> MRGSHHHHHHGRSGDDDDKMKVLNDLLGYKNRKLYQDNKMFNFTLDSVLVARFCNLNS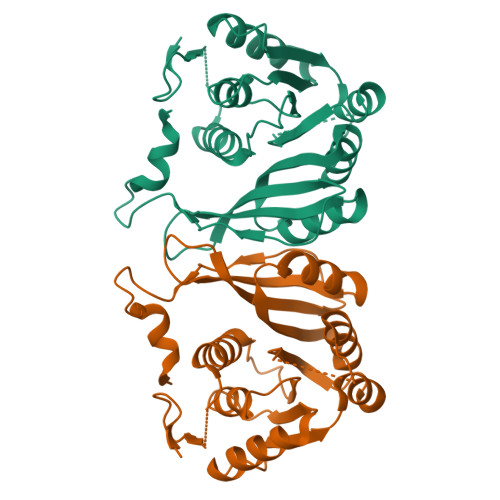KKKKICDFGTNNAVIPLILSKYTKAKIIGVEIQNKAVEIANENIKLNGLEDQIEIVHADIKEFSKLHNQEFDLVVCNPPFFKMDGNPKLKEISLEVANARHEILITLEDIIKSASRCLKNKGNFTIVHRSERLSEIINLFYKYNIYPKRLRLIQSKKTDNAKMILLDGIYQGNEGMEILPTLITHNDDETYTDELLKYFHD>MKVLFLTA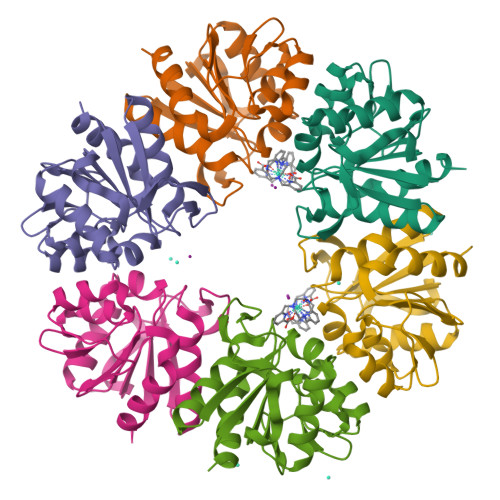NEFEDVELIYPYHRLKEEGHEVYIASFERGTITGKHGYSVKVDLTFDKVNPEEFDALVLPGGRAPERVRLNEKAVSIARKMFSEGKPVASICHGPQILISAGVLRGRKGTSYPGIKDDMINAGVEWVDAEVVVDGNWVSSRVPADLYAWMREFVKLLK[12x]>[2x]GQTPIFDPTVHWLFTTCGASGPHGPTQAQCNNAYQNSNLSVEVGSEGPLKGIQIWKVPATDTYSISGYGAAGGKGGKNTMMRSHGVSVLGIFNLEKDDMLYILVGQQGEDACPSTNQLIQKVCIGENNVIEEEIRVNRSVHEWAGGGGGGGGATYVFKMKDGVPVPLIIAAGGGGRAYGAKTDTFHPERLENNSSVLGLNGNSGAAGGGGGWNDNTSLLWAGKSLQEGA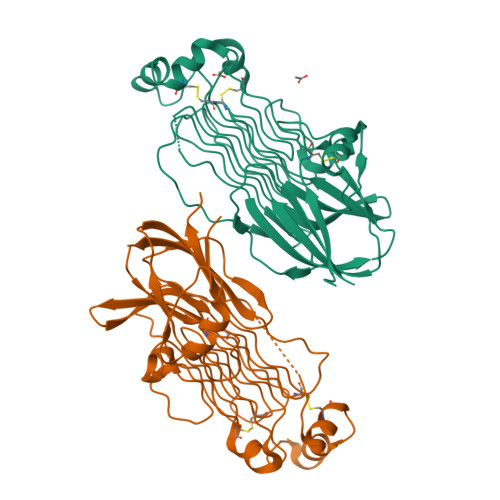TGGHSCPQAMKKWGWETRGGFGGGGGGCSSGGGGGGYIGGNAASNNDPEMDGEDGVSFISPLGILYTPALKVMEGHGEVNIKHYLN> MAHHHHHHDYGIPTTENLYFQGSNPNYCFAGKTSSISDLKEVPRKNITLIRGLGHGAFGEVYEGQVS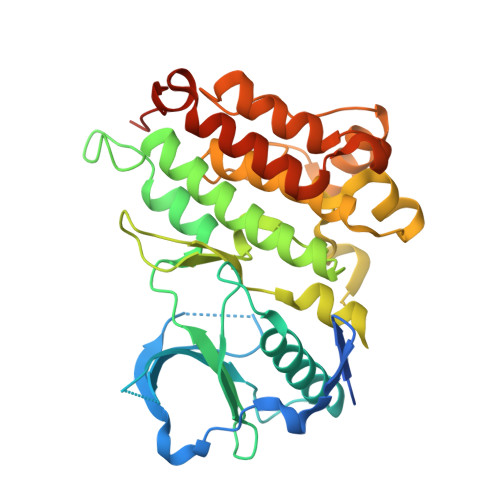GMPNDPSPLQVAVKTLPEVCSEQDELDFLMEALIISKFNHQNIVRCIGVSLQSLPRFILLELMAGGDLKSFLRETRPRPSQPSSLAMLDLLHVARDIACGCQYLEENHFIHRDIAARNCLLTCPGPGRVAKIADFGMARDIYRASYYRKGGCAMLPVKWMPPEAFMEGIFTSKTDTWSFGVLLWEIFSLGYMPYPSKSNQEVLEFVTSGGRMDPPKNCPGPVYRIMTQCWQHQPEDRPNFAIILERIEYCTQDPDVINTALPIEYGPLVEEEEKV> ATGLHVKNGRLYEANGQEFIIRGVSHPHNWYPQHTQAFADIKSHGANTVRVVLSNGVRWSKNGPSDVANVISLCKQNRLICMLEVHDTTGYGEQSGASTLDQAVDYWIELKSVLQGEEDYVLINIGNEPYGNDSATVAAWATDTSAAIQRLRAAGFEHTLVVDAPNWGQDWTNTMRNNADQVYASDPTGNTVFSIHMYGVYSQASTITSYLEHFVNAGLPLIIGEFGH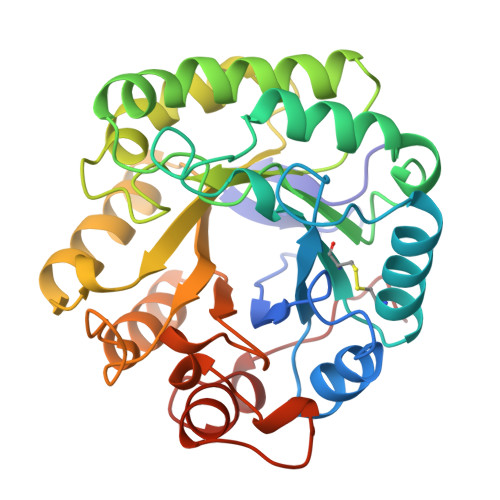DHSDGNPDEDTIMAEAERLKLGYIGWSWSGNGGGVEYLDMVYNFDGDNLSPWGERIFYGPNGIASTAKEAVIFG> GAMEPSAPKELKFGDITKDSVHLTWEPPDDDGGSPLTGYVVEKREVSRKTWTKVMDFVTDLEFTVPDLVQGKEYLFRVCARNKCGPGEPAYVDEPVNMSTPATVPDPPENVKWRDRTANSIFLTWDPPKNDGGSRIKGYIVERCPRGSDKWVACGEPVAETKMEVTGLEEGKWYAYRVKALNRQGASKPSRPTEEIQAV

Titin is a giant, elastic, sarcomeric protein with a molecular weight of more than 3800 kD. Titin consists primarily of two types of protein domains: fibronectin type III (FnIII) domains and immunoglobulin (Ig) domains (ca 100 residues in length) that account for over 90% of its mass. Despite the repetitive composition of titin, a single main immunogenic region (MIR) has so far been identified in its chain that elicits the reactivity of almost all known anti-titin antibodies in MG patients. This 30 kD segment, also termed MGT30, consists of a domain triplet of composition Ig-FnIII-FnIII located in the titin segment at the junction of the I- and A-bands (I/A) and corresponding to domains 4 to 6 in this region of the chain, i.e., tandem I109-I111 also termed I/A4-I/A6, (nomenclature as in Bang et al., 2001).

To gain an insight into the possible molecular determinants of I110 recognition by anti-titin antibodies, we elucidated the 3D-structure of the isolated I110 domain, the double tandem I110-I111 and the full-length MIR region I109-I110 using X-ray crystallography. C-terminally, I110 is joined to the subsequent domain by a flexible three residue long, hydrophilic linker, STA. No direct contacts exist between I110 and I111, so that the linker sequence acts as an effective hinge permitting the free repositioning of both domains. Accordingly, the structures of I110-I111 and I109-I111 show a different mutual arrangement of these domains. The I110 domain showed a stable and same structure when isolated and arrayed with its neighboring domains. The only common element between all MIR protein fragments which were bound to sera in this ELISA screening is the central FnIII domain, I110, suggesting that this domain may contain the binding epitope(s) for anti-titin antibodies in MG patients. The average values of Figure 2B show more clearly that binding to I109-I110, I110-I111 or I110 alone does not significantly differ from their binding to the whole MIR, suggesting that the main binding interface is located in the common element, I110, and that the other domains play no or only a minor role in antibody binding. Importantly, as with the MG sera, binding to domain I110 was very similar to that observed against the full-length MIR tandem, whereas, similarly to the MG sera, practically no serum was bound to domain I111.> XALRGTVTDFSGFDGRADAEVLRKAMKGLGTDEDSILNLLTARSNAQRQQIAEEFKTLFGRDLVNDMKSELTGKFEKLIVALMKPSRLYDAYELKHALKGAGTDEKVLTEIIASRTPEELRAIKQAYEEEYGSNLEDDVVGDTSGYYQRMLVVLLQANRDPDTAIDDAQVELDAQALFQAGELKWGTDEEKFITILGTRSVSHLRRVFDKYMTISGFQIEETIDRETSGNLENLLLAVVKSIRSIPAYLAETLYYAMKGAGTDDHTLIRVIVSRSEIDLFNIRKEFRKNFATSLYSMIKGDTSGDY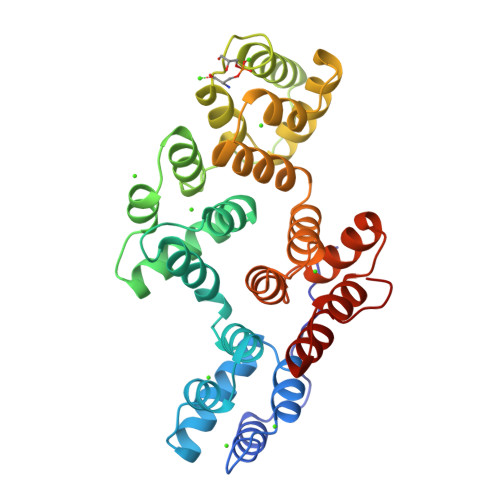KKALLLLCGGEDD> LKGTQSLNPHNDYCQHFVDTGHRPQNFIRDVGLADRFEEYPK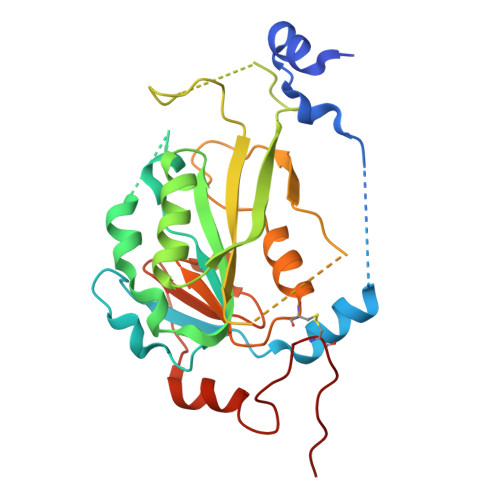LRELIRLKDELIAKSNTPPMYLQADIEAFDIRELTPKFDVILLEPPLEEYYRETGITANEKCWTWDDIMKLEIDEIAAPRSFIFLWCGSGEGLDLGRVCLRKWGYRRCEDICWIKTNKNNPGKTKTLDPKAVFQRTKEHCLMGIKGTVKRSTDGDFIHANVDIDLIITEEPEIGNIEKPVEIFHIIEHFCLGRRRLHLFGRDSTIRPGWLTVGPTLTNSNYNAETYASYFSAPNSYLTGCTEEIERL>SMFLPPPECPVFEPSWAEFRDPLGYIAKIRPIAEKSGICKIRPPADWQPPFAVEVDNFRFTPRIQRLNELEAQTRVKLGGGGGFEQATREYTLQSFGEMADSFKADYFNMPVHMVPTELVEKEFWRLVNSIEEDVTVEYGADIHSKEFGSGFPVSDSKRHLTPEEEEYATSGWNLNVMPVLEQSVLCHINADISGMKVPWLYVGMVFSAFCWHIEDHWSYSINYLHWGEPKTWYGVPSLAAEHLEEVMKKLTPELFDSQPDLLHQLVTLMNPNTLMSHGVPVVRTNQCAGEFVITFPRAYHSGFNQGYNFAEAVNFCTADWLPAGRQCIEHYRRLRRYCVFSHEELICKMAACPEKLDLNLAAAVHKEMFIMVQEERRLRKALLEKGI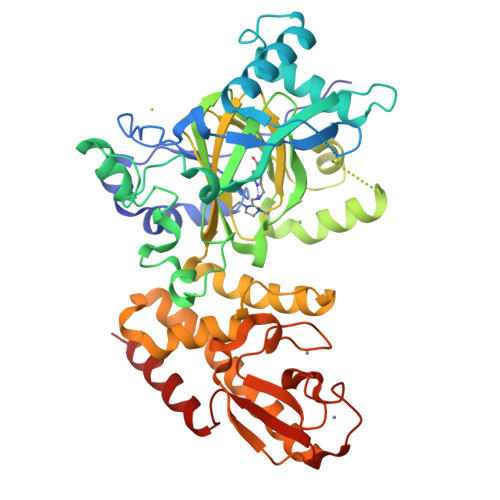TEAEREAFELLPDDERQCIKCKTTCFLSALACYDCPDGLVCLSHINDLCKCSSSRQYLRYRYTLDELPAMLHKLKVRAESFDT[2x]>[4x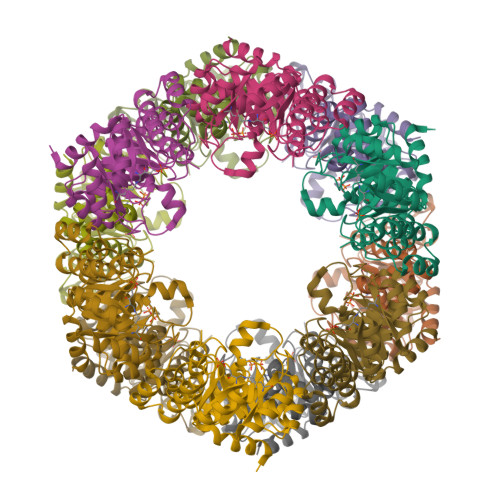]MAGTGVVAVYGEGAMTETKQKSPFSVKVGLAQMLRGGVIMDVVNAEQARIAEEAGACAVMALERVPADIRAQGGVARMSDPEMIKEIKNAVTIPVMAKARIGHFVEAQILEAIGVDYVDESEVLTLADEDNHINKHNFKIPFVCGCRNLGEALRRIREGAAMIRTRGEAGTGNVVEAVRHVRSVNGAIRLLRSMDDDEVFTYAKKIAAPYDLVVQTKELGRLPVVQFAAGGVATPADAALMMQLGCDGVFVGSGVFKSGDPVKRAKAIVQAVTNYRDAAVLAEVSCGLGEAMVGLNLDDKVERFASRSEEHHHHHH The similarity of eukaryotic actin to crenactin, a filament-forming protein from the crenarchaeon Pyrobaculum calidifontis supports the theory of a common origin of Crenarchaea and Eukaryotes. Attempts to trace back the origins of today's eukaryotic F-actin filaments led to the discovery of crenactin found in certain organisms of the order Thermoproteales within the phylum Crenarchaeota (Crenarchaea, part of the 'TACK' superphylum). Hence, it has been proposed that crenactin filaments share a common ancestor with F-actin. In Pyrobaculum calidifontis, crenactin is encoded within the arcade cluster of genes, together with four arcadins, and has been proposed to be part of a cell-shape maintenance system.

Here, we present the near-atomic resolution structure of double-stranded crenactin filaments at 3.8 Å by cryoEM, revealing their close relationship to F-actin. Crenactin forms right-handed, double-stranded, staggered filaments with a rise of 25.6 Å (half a subunits' length, hence staggered) between subunits and a twist of 198.1° (1-start, rotating between the two strands, equivalent to -161.9°). These values are very similar to the parameters of the eukaryotic F-actin filament, with a rise of 27.5 Å and a twist of 193.6° (equivalent to −166.4°). In our filament structure presented here, we observed a dramatic rearrangement of the hydrophobic plug, moving it upwards, towards subdomain IB, by as much as 21 Å. In this new position, the loop interacts extensively with subunits of the opposite strand, essentially the same function as the hydrophobic plug has in F-actin. In addition to the hydrophobic plug, a hydrophilic interaction between subdomain IIB on one strand and subdomain IA on the opposite strand helps to keep the double filament architecture stable. For longitudinal assembly, crenactin subunits within the same strand are held together via three main areas of interactions. Particularly significant is the well-conserved D-loop (DNase I binding loop) located within subdomain IB. Folded into a small alpha helix, it interacts with the previous subunit via a surface usually referred to as the 'hydrophobic groove' in actin. Furthermore, the ATPase active site is also highly conserved with key residues, such as the nucleophilic water activator Q164 (Q137 in actin), in the same place in both structures.

>[6x]MGVISDAYRLKYTFGVDFGTSYVKYGPITLNEPKMVQTRGLFLRDLPESVKMRIPPDVLARGLVVGDEEVRKYLSSVRDVQRNLKYPLKDGVARRDDEEAWRVLKELARYTLAQFPVSDPEFAGWLVAVALSALAPDYMYKAIFDIYDELASEFKIYAVTILPQPLAVAIAENAVNCVIVEGGHGNIQVAPISFALIREGLVALNRGGAEANAITREILKDIGYSDIAREEYAVEVVKRAVGLVPRRLKEAIRAAKSDPDRFVTKVRLSPVVEVEIPREYAWTRFLIGEIVFDPNHEEIKSYIEQSRLRIENAVIGDVTLYGEMDVASAIITSLRNVSVEIQERVASQIILSGGAFSWRVPPGMEDVAADSVTRVKIALEEKSPALASKVEVRLVSEPQYSVWRGAVIYGYALPLSLEWSDTTREGWRFPRR>HHHHHHSDSQQSIKVLEELFQKLSVATADNRHEIASEVASFLNGNIIEHDVPEHFFGELAKGIKDKKTAANAMQAVAHIANQSNLSPSVEPYIVQLVPAICTNAGNKDKEIQSVASETLISIVNAVNPVAIKALLPHLTNAIVETNKWQEKIAILAAFSAMVDAAKDQVALRMPELIPVLSETMWDTKKEVKAAATAAMTKATETVDNKDIERFIPSLIQCIADPTEVPETVHLLGATTFVAEVTPATLSIMVPLLSRGLNERETGIKRKSAVIIDNMCKLVEDPQVIAPFLGKLLPGLKSNFATIADPEAREVTLRALKTLRRVGNVGEDDAIPELSHAGDVSTTLQVVNELLKDETVAPRFKIVVEYIAAIGADLIDERIIDQQAWFTHITPYMTIFLHEKKAKDILDEFRKRAVDNIPVGPNFDDEEDEGEDLCNCEFSLAYGAKILLNKTQLRLKRARRYGICGPNGCGKSTLMRAIANGQVDGFPTQEECRTVYVEHDIDGTHSDTSVLDFVFESGVGTKEAIKDKLIEFGFTDEMIAMPISALSGGWKMKLALARAVLRNADILLLDEPTNHLDTVNVAWLVNYLNTCGITSITISHDSVFLDNVCEYIINYEGLKLRKYKGNFTEFVKKCPAAKAYEELSNTDLEFKFPEPGYLEGVKTKQKAIVKVTNMEFQYPGTSKPQITDINFQCSL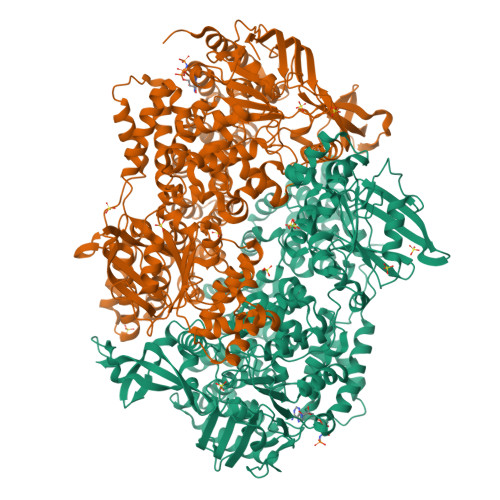SSRIAVIGPNGAGKSTLINVLTGELLPTSGEVYTHENCRIAYIKQHAFAHIESHLDKTPSEYIQWRFQTGEDRETMDRANRQINENDAEAMNKIFKIEGTPRRIAGIHSRRKFKNTYEYECSFLLGENIGMKSERWVPMMSVDNAWIPRGELVESHSKMVAEVDMKEALASGQFRPLTRKEIEEHCSMLGLDPEIVSHSRIRGLSGGQKVKLVLAAGTWQRPHLIVLDEPTNYLDRDSLGALSKALKEFEGGVIIITHSAEFTKNLTEEVWAVKDGRMTPSGHNWVSG[2x]>[6x]GARSVRTTRGKRKRVDVEESEASSSVSISHSASATGN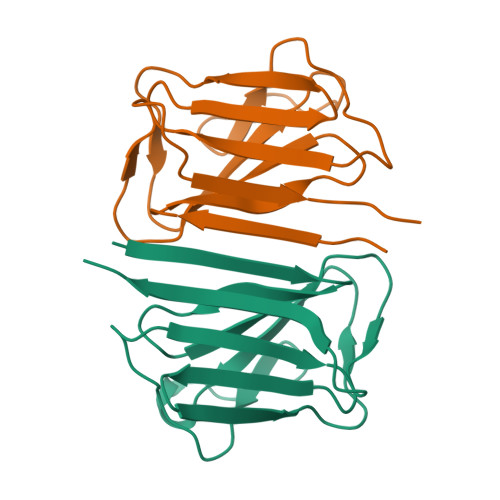VCIEEIDVDGKFIRLKNTSEQDQPMGGWEMIRKIGDTSVSYKYTSRYVLKAGQTVTIWAANAGVTASPPTDLIWKNQNSWGTGEDVKVILKNSQGEEVAQRSTVFKTTIPEE>[2x]TDTFQMFWLDYCEVNNTLILFGKVKLKDDNCVSAMVQINGLCRELFFLPREGKTPTDIHEEIIPLLMDKYGLDNIRAKPQKMKYSFELPDIPSESDYLKVLLPYQTPKSSRDTIPSDLSSDTFYHVFGGNSNIFESFVIQNRIMGPCWLDIKGADFNSIAAASHCAVEVSVDKPQNITPTTTKTMPNLRCLSLSIQTLMNPKENKQEIVSITLSAYRNISLDSPIPENIKPDDLCTLVRPPQSTSFPLGLAALAKQKLPGRVRLFNNEKAMLSCFCAMLKVEDPDVIIGHRLQNVYLDVLAHRMHDLNIPTFSSIGRRLRRTWPEKFGRGNSNMNHFFISDICSGRLICDIANEMGQSLTPKCQSWDLSEMYQVTCEKEHKPLDIDYQNPQYQNDVNSMTMALQENITNCMISAEVSYRIQLLTLTKQLTNLAGNAWAQTLGGTRAGRNEYILLHEFSRNGFIVPDKEGNRSRAQKQRQNEENADAPVNSKKAKYQGGLVFEPEKGLHKNYVLVMDFNSLYPSIIQEFNICFTTVDRNKEDIDELPSVPPSEVDQGVLPRLLANLVDRRREVKKVMKTETDPHKRVQCDIRQQALKLTANSMYGCLGYVNSRFYAKPLAMLVTNKGREILMNTRQLAESMNLLVVYGDTNSVMIDTGCDNYADAIKIGLGFKRLVNERYRLLEIDIDNVFKKLLLHAKKKYAALTVNLDKNGNGTTVLEVKGLDMKRREFCPLSRDVSIHVLNTILSDKDPEEALQEVYDYLEDIRIKVETNNIRIDKYKINMKLSKDPKAYPGGKNMPAVQVALRMRKAGRVVKAGSVITFVITKQDEIDNAADTPALSVAERAHALNEVMIKSNNLIPDPQYYLEKQIFAPVERLLERIDSFNVVRLSEALGLDSKKYFRREGGNNNG

The eukaryotic primase is a heterodimer of catalytic and regulatory subunits that is associated with the catalytic subunit of Pol α and its accessory B subunit in a constitutive heterotetrameric assembly, the Pol α/primase complex. In contrast, the Pol α/primase complex produces longer, composite RNA-DNA primers that result from the concerted enzymatic activities of primase and Pol α (Chang et al., 1984; Hu et al., 1984; Singh, et al., 1986). We have determined crystal structures of the catalytic core (349–1258; 910 amino acids) of yeast Pol α in unliganded form (apo), bound to an RNA primer/DNA template duplex (binary complex) and in a productive complex with RNA primer/DNA template and incoming dGTP (ternary complex). The catalytic region of Pol α adopts the universal ‘right-hand' DNA polymerase fold consisting of a palm domain harboring the active site, a fingers domain that interacts with the incoming nucleotide and a thumb domain that grips the primer-template duplex.

For structural studies of the ternary complex, we used a polymerase mutant (D998N) with attenuated catalytic activity. During crystallization of the ternary complex, the polymerase extended the 3′-end of the RNA primer by addition of two deoxyguanosine nucleotides. The RNA primer–DNA template helix bound to Pol α adopts overall an A-DNA conformation. The majority of the contacts of the polymerase with the primer/template duplex takes place within a region of 7 bp from the 3′-terminus of the templated primer. The interactions between the thumb domain and the RNA primer are concentrated in a contiguous region of five nucleotides, from position two to six of the RNA primer and involve solely the ribose and phosphate moieties of the RNA backbone. Pol α exploits the wide, shallow nature of the minor groove of the RNA/DNA helix with a series of hydrophobic contacts involving the side chains of Met1131, Leu1133, Tyr1140, Pro1141, Met1146, which recognize the C3′-endo conformation of the ribose moieties of RNA nucleotides in position four to six. The contiguous pair of invariant arginine residues 1075 and 1076 straddles the ribose-phosphate backbone between nucleotides three and four from the 3′-end of the RNA primer. The side chain of Arg1075 extends into the minor groove and packs its guanidinium moiety against the ribose sugar of Ade4, thus engaging in an interaction that matches closely the contact made by the equivalent Arg839 of yeast Pol δ with the DNA primer. However, in the case of Pol α the close contact with Arg1075 induces a local rearrangement of the RNA conformation, which includes a B-DNA C2′-endo ribose pucker for Ade4 and unstacking between the aromatic bases of nucleotides four and five. The local conformation of the RNA primer is stabilized by insertion of the Arg1076 side chain between the phosphate groups of nucleotides three and four.>RSYEQMETDGERQNATEIRASVGKMIDGIGRFYIQMCTELKLSDYEGRLIQNSLTIERMVLSAFDERRNKYLEEHPSAGKDPKKTGGPIYRRVDGKWRRELILYDKEEIRRIWRQANNGDDATAGLTHMMIWHSNLNDATYQRTRALVRTGMDPRMCSLMQGSTLPRRSGAAGAAVKGVGTMVMELIRMIKRGINDRNFWRGENGRRTRIAYERMCNILKGKFQTAAQRTMVDQVRESRNPGNAEFEDLIFLARSALILRGSVAHKSCLPACVYGSAVASGYDFEREGYSLVGIDPFRLLQNSQVYSLIRPNENPAHKSQLVWMACHSAAFEDLRVSSFIRGTKVVPRGKLSTRGVQIASNENMETMESSTLELRSRYWAIRTRSGGNTNQQRASS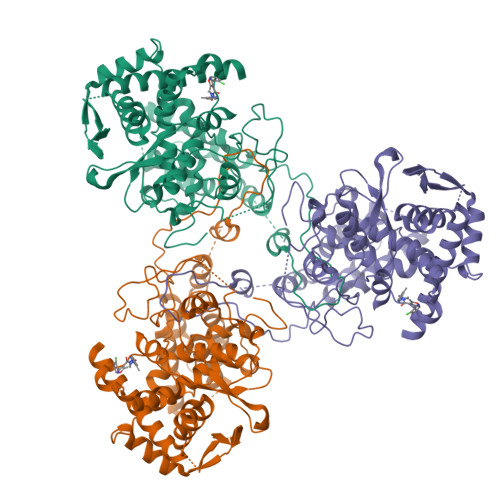GQISIQPTFSVQRNLPFDRPTIMAAFTGNTEGRTSDMRTEIIRLMESARPEDVSFQGRGVFELSDEKATSPIVPSFDMSNEGSYFFGDNAEEYDNLEHHHHHH[2x]>[4x]DSARSFLERLEARGGREGAVLAGEFSDIQACSAAWKADGVCSTVAGSRPENVRKNRYKDVLPYDQTRVILSLLQEEGHSDYINGNFIRGVDGSLAYIATQGPLPHTLLDFWRLVWEFGVKVILMACREIENGRKRCER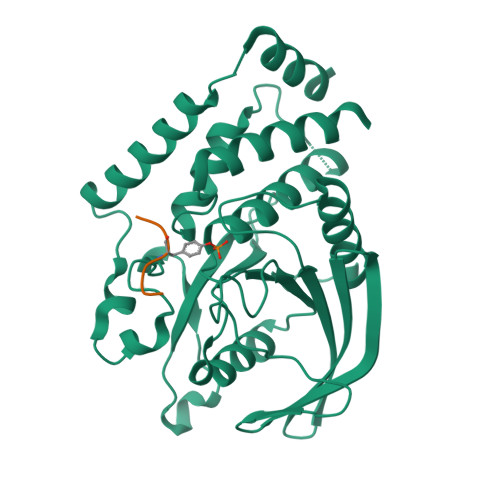YWAQEQEPLQTGLFCITLIKEKWLNEDIMLRTLKVTFQKESRSVYQLQYMSWPDRGVPSSPDHMLAMVEEARRLQGSGPEPLCVHSSAGCGRTGVLCTVDYVRQLLLTQMIPPDFSLFDVVLKMRKQRPAAVQTEEQYRFLYHTVAQMFCST;>[4x]LQRYSE>[4x]MAVLGLQGVRGGVGTTTITAALAWSLQMLGENVLVVDACPDNLLRLSFNVDFTHRQGWARAMLDGQDWRDAGLRYTSQLDLLPFGQLSIEEQENPQHWQTRLSDICSGLQQLKASGRYQWILIDLPRDASQITHQLLSLCDHSLAIVNVDANCHIRLHQQALPDGAHILINNFRIGSQVQDDIYQLWLQSQRRLLPMLIHRDEAMAECLAAKQPVGEYRSDALAAEEILTLANWCLLNYSGLKTPVGSKS;>[4x]GPMGSMNNNEPDTLPDPAIGYIFQNDIVALKQAFSLPDIDYADISQREQLAAALKRWPLLAEFAQQK;>[4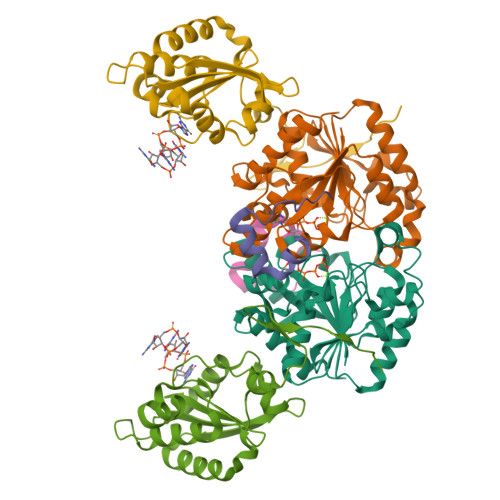x]MGSMEDITTLLSMTQPLKLRGFQKWDVFCNAVNNMMNNPLLPAHGKGVLVALRPVPGIRVEQALTLCRPNRTGDIMTIGGNRLVLFLSFCRINDLDTALNHIFPLPTGDIFSNRMVWFEDDQISAELVQMRLLAPEQWGMPLPLTQSSKPVINAEHDGRHWRRIPEPMRLLDDAVERSS>[2x]MVAIIFDMDGVLYRGNRAIPGVRELIEFLKERGIPFAFLTNNSTKTPEMYREKLLKMGIDVSSSIIITSGLATRLYMSKHLDPGKIFVIGGEGLVKE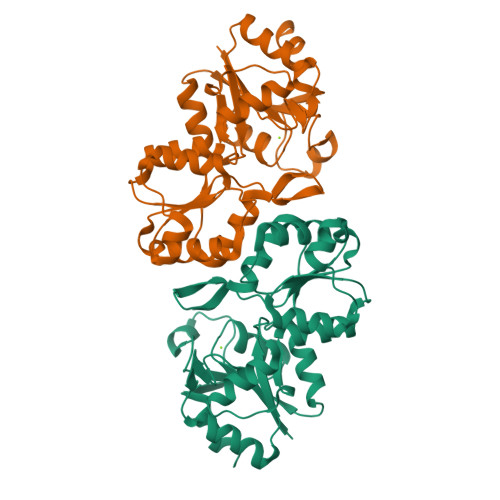MQALGWGIVTLDEARQGSWKEVKHVVVGLDPDLTYEKLKYATLAIRNGATFIGTNPDATLPGEEGIYPGAGSIIAALKVATNVEPIIIGKPNEPMYEVVREMFPGEELWMVGDRLDTDIAFAKKFGMKAIMVLTGVSSLEDIKKSEYKPDLVLPSVYELIDYLKTL>[4x]SNAHKGTLYVVATPLGNLDDMTFRAVNTLRNAGAIACEDTRR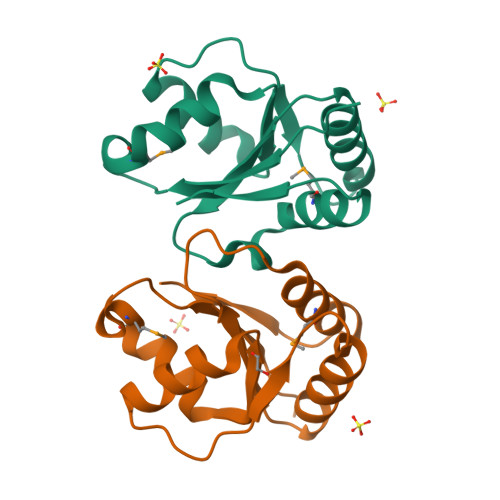TSILLKHFGIEGKRLVSYHSFNEERAVRQVIELLEEGSDVALVTDAGTPAISDPGYTMASAAHAAGLPVVPVPGA> GPHMGGSMAEPVSPLKHFVLAKKAITAIFDQLLEFVTEGSHFVEATYKNPELDRIATEDDLVEMQGYKDKLSIIGEVLSRRHMKVAFFGRTSSGKSSVINAMLWDKVLPSGIGHITNCFLSVEGTDGDKAYLMTEGSDEKKSVKTVNQLAHALHMDKDLKAGCLVRVFWPKAKCALLRDDLVLVDSPGTDVTTELDSWIDKFCLDADVFVLVANSESTLMNTEKHFFHKVNERLSKPNIFILNNRWDASASE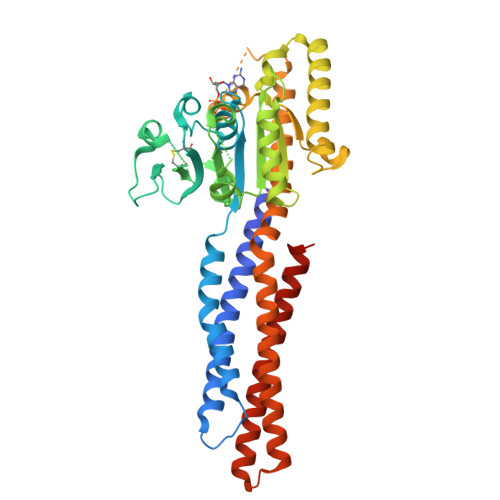PEYMEDVRRQHMERCLHFLVEELKVVNALEAQNRIFFVSAKEVLSARKQKAQGMPESGVALAEGFHARLQEFQNFEQIFEECISQSAVKTKFEQHTIRAKQILATVKNIMDSVNLAAEDKRHYSARLPKEIDQLEKIQNNSKLLRNKAVQLENELENFTKQFLPSSNEES>HHHHHHSSGLVPRGSHMENPLQKARILVNQLEKYLDRYAKEYDVEHLAGPQGHLVMHLYKHPDKDMSIKDAEEILHISKSVASNLVKRMEKNGFIAIVPSKTDKRVKYLYLTHLGKQKATQFEIFLEKLHSTMLAGITKEEIRTTKKVIRTLAKNMAMEDFD[4x]

In the present study, we conducted structural and functional analyses of the heme-responsive sensor protein PefR (porphyrin-regulated efflux regulator) from the β-hemolytic bacterium Streptococcus agalactiae, which is the most common cause of life-threatening invasive bacterial infections (e.g., septicemia, pneumonia, and meningitis) during the neonatal period. Therefore, PefR promotes the expression of these heme efflux systems in S. agalactiae in response to the intracellular heme concentration, likely by binding heme. The monomer consists of six α-helices and two β-strands containing a winged helix-turn-helix (wHTH) motif. This architecture of PefR is similar to that of the multiple antibiotic resistance regulator (MarR) family of transcriptional regulators, in which helices α2–α4 and strands β1–β2 form the DNA-binding domains.

Recombinant PefR was purified in its apo form. Gel filtration analyses showed that apo-PefR eluted as a single peak with an estimated molecular mass of ~35 kDa, indicating that PefR (ca. 17 kDa in monomer) exists as a homodimer in solution. We observed structural distortions by the N-terminal His tag by comparing the X-ray crystal structures of apo-PefR with and without the N-terminal His tag.> GSMVKSQKVIDVLNAHYNLNLELGSVYAQYAHIADDQFSMPFLAKFINDLSNDKLGVHKDLISEYARKIEIPLHTKFSVDVSFKPTDPKELVKHILETEQKVRKHVANMAKVCL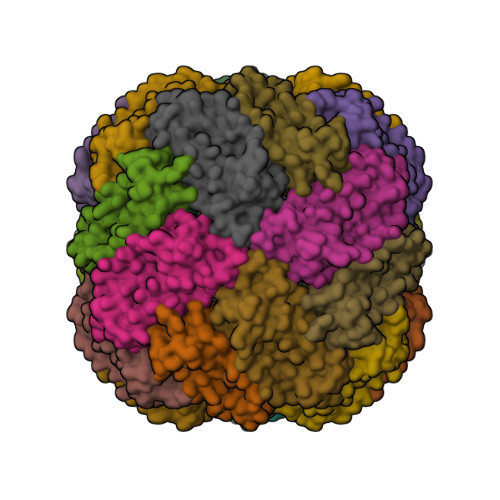EEGDFETFSFVKWFVDDGIKDFDDVRTIHDFFENGNNNLQVEYAIRKYLKQMKLEEEK>MKHGIYYAYWEKQWQADYIPYIEKAAQLGFDILEIAASPLPFYSEQQMKDIKACAEANGITLTCGHGPSPDQNLASSDPAVRAHAKSFFTDLLSRLEKMDIHVIGGGIYSYWPVDYSMPIDKPGDWARSVEGVAEMAKVAESCGVDYCLEVLNRFEGYLLNTAEEAVQFVQEVNHPRVKIMLDTFHMNIEEDSIGG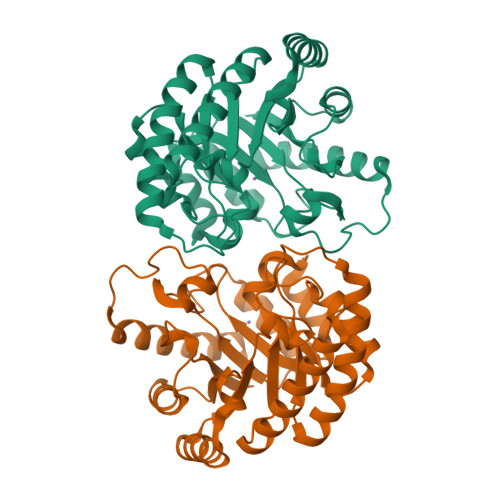AIRRAGQHLGHFHTGECNRRVPGRGRTPWREIGEALRDIGYTGAVVMEPFVRMGGQVGSDIKIWREMNPGADDAQLDLDAKNAVTFQRYMLD[2x]> MMNEKILIVDDQSGIRILLNEVFNKEGYQTFQAANGLQALDIVTKERPDLVLLDMKIPGMDGIEILKRMKVIDENIRVIIMTAYGELDMIQESKELGA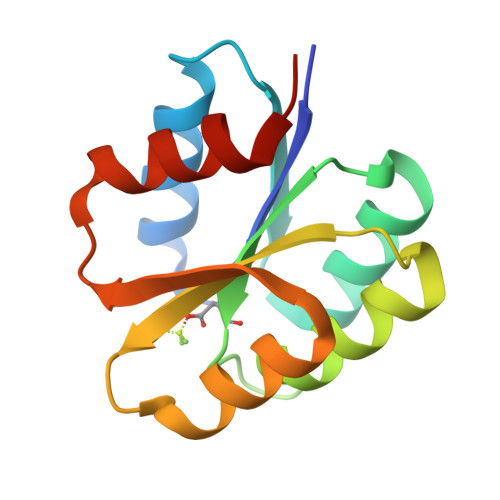LTHFAKPFDIDEIRDAVKKYLPLKSN> SDPITGGHYENHNGYFVYIDASGKQVTGLQNIDGNLQYFDDNGYQVKGSFRDVNGKHIYFDSVTGKASSNVDIVNGKAQGYDAQGNQLKKSYVADSSGQTYYFDGNGQPLIGLQTIDGNLQYFNQQGVQIKGGFQDVNNKRIYFAPNTGNAVANTEIINGKLQGRDANGNQVKNAFSKDVAGNTFYFDANGVMLTGLQTISGKTYYLDEQGHLRKNYAGTFNNQFMYFDADTGAGKTAIEYQFDQGLVSQSNENTPHNAAKSYDKSSFENVDGYLTADTWYRPTDILKNGDTWTASTETDMRPLLMTWWPDKQTQANYLNFMSSKGLGITTTYTAATSQKTLNDAAFVIQTAIEQQISLKKSTEWLRDAIDSFVKTQANWNKQTEDEAFDGLQWLQGGFLAYQDDSHRTPNTDSGNNRKLGRQPINIDGSKDTTDGKGSEFLLANDIDNSNPIVQAEQLNWLHYLMNFGSITGNNDNANFDGIRVDAVDNVDADLLKIAGDYFKALYGTDKSDANANKHLSILEDWNGKDPQYVNQQGNAQLTMDYTVTSQFGNSLTHGANNRSNMWYFLDTGYYLNGDLNKKIVDKNRPNSGTLVNRIANSGDTKVIPNYSFVRAHDYDAQDPIRKAMIDHGIIKNMQDTFTFDQLAQGMEFYYKDQENPSGFKKYNDYNLPSAYAMLLTNKDTVPRVYYGDMYLEGGQYMEKGTIYNPVISALLKARIKYVSGGQTMATDSSGKDLKDGETDLLTSVRFGKGIMTSDQTTTQDNSQDYKNQGIGVIVGNNPDLKLNNDKTITLHMGKAHKNQLYRALVLSNDSGIDVYDSDDKAPTLRTNDNGDLIFHKTNTFVKQDGTIINYEMKGSLNALISGYLGVWVPVGASDSQDARTVATESSSSNDGSVFHSNAALDSNVIYEGFSNFQAMPTSPEQSTNVVIATKANLFKELGITSFELAPQYRSSGDTNYGGMSFLDSFLNNGYAFTDRYDLGFNKADGNPNPTKYGTDQDLRNAIEALHKNGMQAIADWVPDQIYALPGKEVVTATRVDERGNQLKDTDFVN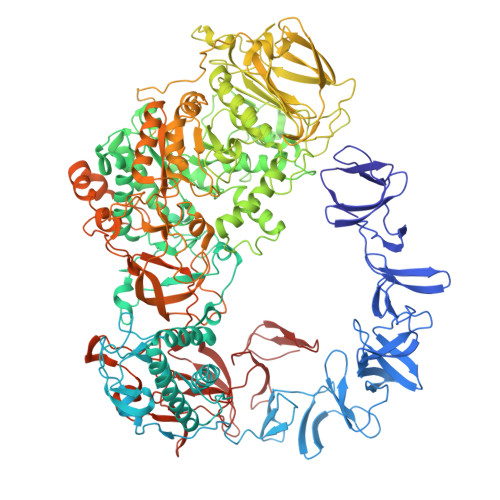LLYVANTKSSGVDYQAKYGGEFLDKLREEYPSLFKQNQVSTGQPIDASTKIKQWSAKYMNGTNILHRGAYYVLKDWATNQYFNIAKTNEVFLPLQLQNKDAQTGFISDASGVKYYSISGYQAKDTFIEDGNGNWYYFDKDGYMVRSQQGENPIRTVETSVNTRNGNYYFMPNGVELRKGFGTDNSGNVYYFDDQGKMVRDKYINDDANNFYHLNVDGTMSR SAP05 is an effector from a plant pathogenic phytoplasma that mediates the degradation of host transcription factors, including SPL and GATA family proteins, by hijacking the 26 S plant ubiquitin receptor RPN10 independently of substrate ubiquitination. Specifically, SAP05 folds into a tight globular structure consisting of a parallel five-stranded β-sheet (β1-β5). Although SAP05 carries a single domain, it utilizes two opposing surfaces (hereafter referred to as Lobe1 and Lobe2) to interact simultaneously with TFs and AtRPN10, forming a dumbbell-shaped structure, in which TFs and AtRPN10 have no direct surface contacts. In summary, SAP05 bridges the TFs mainly through electrostatic interactions with a hydrophobic core, whereas the SAP05-AtRPN10 interface comprises predominantly extensive hydrophobic contacts.

In the SAP05-GATA18 binary complex, the ZnF of GATA18 has a type IV zinc finger motif containing a single zinc CysX2CysX18CysX2Cys zinc finger, in which the zinc ion is chelated by four cysteine residues (Cys154, Cys157, Cys176 and Cys179) located on the α-helix and the extended loop. This zinc finger motif is evolutionarily conserved from plants to animals. Upon inspection of the complex structures, we found that the Lobe1 of SAP05 creates an acidic surface that interacts with the complementary basic surface of TFs. For instance, in the SAP05-GATA18 structure, the guanidine group of Arg188 from GATA18 forms a bidentate salt bridge with the carboxyl group of Asp106 from SAP05. Simultaneously, the Lys185 of GATA18 is salt-bridged to the negatively charged Asp106 and Glu107 of SAP05. Furthermore, Arg182 of GATA18 forms another bidentate salt bridge with Asp108 of SAP05. Apart from electrostatic interactions, the α-helix of GATA18 is further stabilized through hydrophobic interaction between Ile181 of GATA18 and Ile84-Trp85 of SAP05. At the edge of the α-helix of GATA18, the side-chain carboxamide of Asn177 is coordinated by two hydrogen bonds with the carboxyl group of Asp66 and the backbone carbonyl of Phe81 from SAP05. In the SAP05-GATA18 interface, three pairs of salt-bridge interactions stabilize this binary complex, whereas a single alanine mutation of the negatively charged residue (Asp106, Glu107 or Asp108) in SAP05 or the positively charged residue (Arg182, Lys185 or Arg188) in GATA18 diminished the binding affinity by 3- to 40-fold. Through sequence alignment and structural analysis of AtGATA and leafhopper vector MqGATA (Macrosteles quadrilineatus), we found that the three positively charged residues Arg182, Lys185 and Arg188 in AtGATA, which form multiple salt bridges with SAP05, are not conserved in MqGATA.

>[2x]GDSLLARRCANCDTTSTPLWRNGPRGPKSLCNACGIRFKKEERRTTAATGNT;>[2x]GAPHEERVGDMRIVNITFSDINSIKNFQPFSQYFDFTLTGPRYNGNIAQFAMIWKIKNPPHNLLGVFFDNNTRDDEDDKYTLEELKQMGNGAKNMYIFWQYEQK>MVLYFIGLGLYDERDITCKGLEIAKKCDYVFAEFYTSLMAGTTLGRIQKLIGKEIRVLSREDVELNFENIVLPLAKENDVAFL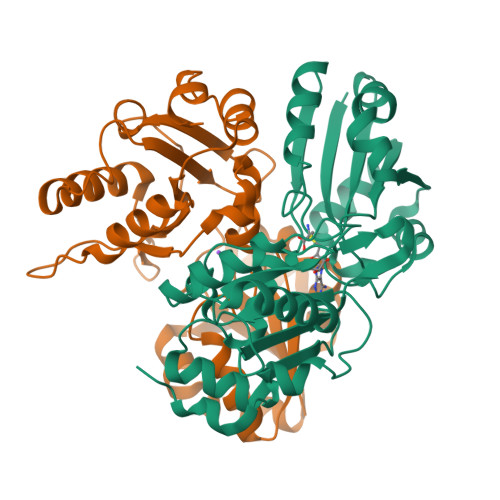TPGDPLVATTHAELRIRAKRAGVESYVIHAPSIYSAVGITGLHIYKFGKSATVAYPEGNWFPTSYYDVIKENAERGLHTLLFLDIKAEKRMYMTANEAMELLLKVEDMKKGGVFTDDTLVVVLARAGSLNPTIRAGYVKDLIREDFGDPPHILIVPGKLHIVEAEYLVEIAGAPREILRVNV[2x]>SMAPTKPKNKSKKSKDRARLKVASSQTSINPKELLDRATTLLEEGDIETAAKVARTAYEHIGENGRHAGAALTLLGQIHVELGDIDAARNYYAAAVKVDEDGSLPEELGGGPEKFLWLAQLSEEGGHDSVAW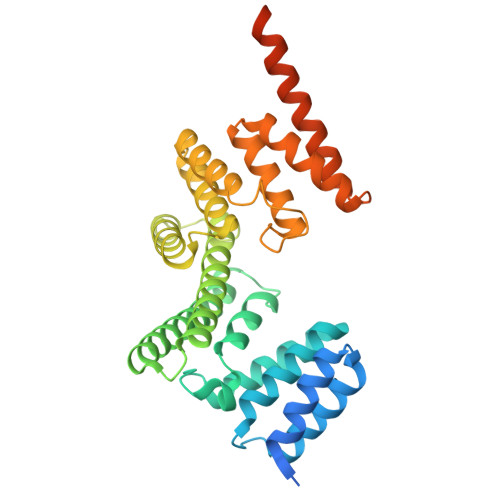FERGATVLRAQIQSLMDSLEQRPLSRGQVEAAIADKRRRLAETLCAVVEVYMTDLSWEDDAEQRCEALITEATMIAPEWPETWQTVANVRISQERTEEAREALRRSLGLWTHLPPEDPGVPPFPSRVSLVRLLIEVDMEEEALEVTERLIAEDDLSVEVWYLGGYARYRLGEKEREASGQASEPEAWKDTWRSSRKWLRQCLKVFEA[2x]> MTALTESSTSKFVKINEKGFSDFNIHYNEAGNGETVIMLHGGGPGAGGWSNYYRNVGPFVDAGYRVILKDSPGFNKSDAVVMDEQRGLVNARAVKGLMDALDIDRA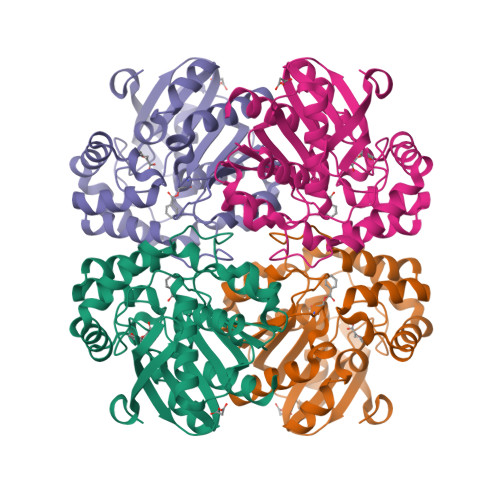HLVGNSMGGATALNFALEYPDRIGKLILMGPGGLGPSMFAPMPMEGIKLLFKLYAEPSYETLKQMLQVFLYDQSLITEELLQGRWEAIQRQPEHLKNFLISAQKAPLSTWDVTARLGEIKAKTFITWGRDDRFVPLDHGLKLLWNIDDARLHVFSKCGQWAQWEHADEFNRLVIDFLRHA methyl 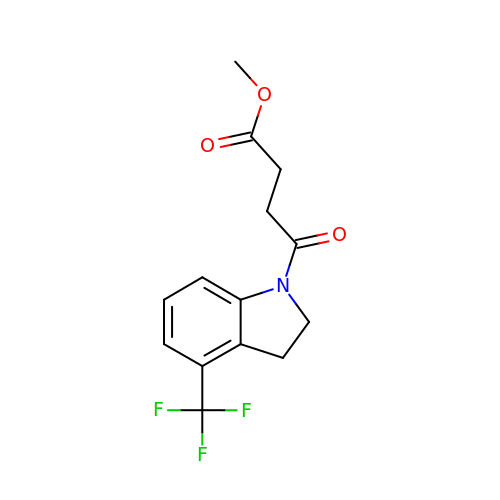4-oxidanylidene-4-[4-(trifluoromethyl)-2,3-dihydroindol-1-yl]butanoate | C14 H14 F3 N O3 | ZCVAYWXZXDNCFC-UHFFFAOYSA-N> NNDDPVENFVESTLKEVLVVPDTKPSGPQHTTKPSILGAMEIGASSNATPESTIETRYVYNTNTNAEADVEMFLGRSALWGKVTLTRQYAKWEINFQEQAHIRKKFEFFTYLRFDM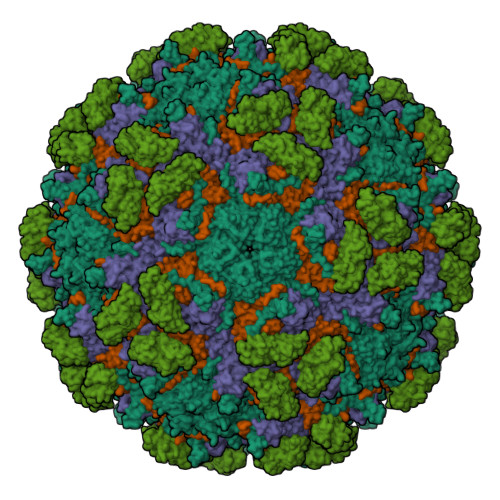EVTIVTNNKGLMQIMFVPPGIDHPETHDDRKWDSASNPSVFFQPKSGFPRFTIPFTGLASAYYMFYDGYDKPKGSDNNEYGIAPTNDMGLLCFRTLDNSGGNDVKIYVKPKHITAWVPRPPRATQYTHKYSTNYHYKPNSSGPDEHVLKDRHFIKTRPLISSA;> GLPTRLPSGSQQFMTTEDEQSPNILPGFHPSKKIHIPGMITNVMHMARVDSFIPINNIQGEVGKVSMYYITVTKKTVTERILVLPLEMSNTLFATTLLGEVLNYYANWSGSITITFMCVCDAFSTGKFLVAYTPPGGKLPEDRKQAMLGVHIIWDLGLQSSCTIVVPWISSGFYRRTKADSFTHGGYVSLWYQTAFVPPVSGGTGSILATCSACPDMSVRMLRDSPMMEQKNELQ;> SPSVEACGYSDRLKQITIGNSTITTQDSLHTVLAYGEWPTYLSDIDATSVDKPTHPETSADRFYTLDSVEWQVGSHGWWWKLPDALKDMGVFGQNMYYHSMGRSGFIIHTQCNATKFHSGALIVAVIPEHQLAYVGGVKVNVGYDHTHPGQSGHQIRGPSQSNDRSGGKPDEDPLFNCNGTLLGNITIFPHQIINLRTNNSSTIVVPYINCVPMDNMLKHNNLSLVIIPLVPLRPGSSGINSVPITVTIAPYKSEFSGAMEAQRQ;> GAQVSRQNNGTHENGVTASNGSVIKYFNINYYKDSASSGLSRQDFSQDPSKFTQPLVDTLTNPALM;> MASDYKDDDDKLHLILLPATGNVAENSPPGTSVHKFSVKLSASLSPVIPGFPQIVNSNPLTEAFRVNWLSGTYFEVVTTGMEQLDFETGPNIFDLQIYVKDEVGVTDLQVLTVQVTDVNEPPGGTKHHHHHH>[12x]MRDSNNIKYVREDAKKMHKLWAHIRMAMEGSRAIKDNAKEFVPHPDNTKATTPEGVARYKAYIERAVWYGASANTVDGMLGQIFARDPVFTGPEDKFDMLINDVDGSGLSIHQQARDSAEDALSLGRGGLFVDYSYVTTNGVSEAQEESGEARPYIKFIAAEDILNWRERWVNGAKRTTLLVFREESDADDDGYQIYKEEVWRELRLVDGTYWQRTWRENDGQLYVDDWISPTKADGSQFDEIPFVIFGSKNNDPTIDMPPMRDLVELNIAHFRNSADYEEACFICGQPTLFLSGLTEHWVKNVLGGAVVIGSRDAVPLPVNAKPELLQAEGNGMVKEAMDQKERQMVALGAKLIDSDKTQRTFG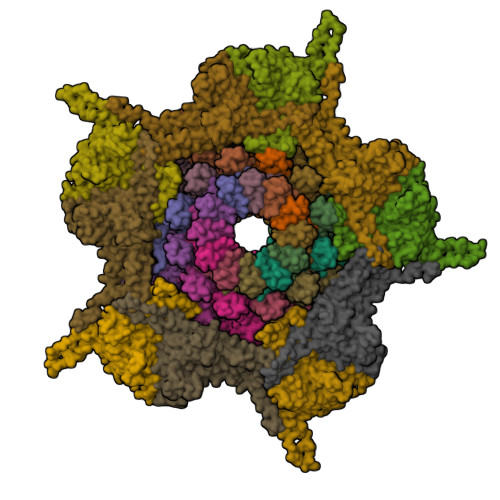EASMEAAAQNSVLSRVSKNVSDAYTKALRWAAMFLGLDEKIEYELNSDFDINKMSPEELAAVISAWQSNAISFTEMRWQIKKGGRAYLEDEDMRNESEQDDPLKLDITKPDPNEDPNASEDDQTDPNDETKEKDAETGGAE;>[10x]MALSDLQVFNDWAYKTMSEVLDQQVELFNGATRGAIILRSAGNTGDLSEAAFWAKIQGLVRPRDPYSNADVAAKDLRQLVDNTIKVASGTPPINIPPSMLRWIQKNPQEAGAVIGQQLAGDTMQDMLNNGLAAGKAAFTAGGAVHDISAAGTGLMTQRAFNAAQRIFGDRSTDIQVWVSHSSPLFDLYDNALANAEQLYVFGTVNVRADAFGRPIIITDSPALVSGAAETLRHSTLGLTTGAILIEQNQDFDSTVVDGTGKQNITRQYQAEWSYNLGVNGYAYDIATGGKAPNPTALATAANWDKISTSIKDTGGVVLVTK In contrast to the majority of carbapenemases, OXA-48-like carbapenemases have low activity toward carbapenems and show no significant hydrolysis of extended-spectrum cephalosporins, including CAZ. Here, we report the occurrence of single (OXA-48:P68A) and double (OXA-48:P68A,Y211S) amino acid substitutions within OXA-48 as a response to CAZ and CAZ-AVI exposure, respectively. The antimicrobial susceptibility data and enzyme kinetics showed that the P68A substitution was responsible for an increased activity toward CAZ, whereas P68A,Y211S led to a decrease in the inhibitory activity of AVI. X-ray crystallography structures revealed that OXA-48:P68A leads to increased flexibility within the OXA-48 structure, likely contributing to elevated CAZ hydrolysis.

Two new crystal structures of OXA-48:P68A were obtained after soaking. The second OXA-48:P68A structure was in complex with AVI (OXA-48:P68A-AVI) and resolved to 2.22 Å. Furthermore, we found AVI covalently bound to S70 in all OXA-48:P68A-AVI chains. R214 and the Ω-loop were in the same conformation as in the native OXA-48. For OXA-48:P68A, we observed no change in the inhibitory activity of AVI. In addition, Y211 in OXA-48 stabilizes AVI binding by aromatic stacking. In addition, S211 contributes to the reduced inhibitory activity of AVI by the loss of aromatic stacking, which stabilizes AVI in OXA-48 and OXA-48:P68A.

>[4x]MRVLALSAVFLVASIIGMPAVAKEWQENKSWNAHFTEHKSQGVVVLWNENKQQGFTNNLKRANQAFLAASTFKIPNSLIALDLGVVKDEHQVFKWDGQTRDIATWNRDHNLITAMKYSVVPVYQEFARQIGEARMSKMLHAFDYGNEDISGNVDSFWLDGGIRISATEQISFLRKLYHNKLHVSERSQRIVKQAMLTEANGDYIIRAKTGYSTRIEPKIGWWVGWVELDDNVWFFAMNMDMPTSDGLGLRQAITKEVLKQEKIIP>[6x]MDRPAVAGPMDLPIMHDSDRYELVKDIGAGNFGVARLMRDKQANELVAVKYIERGEKIDENVKREIINHRSLRHPNIVRFKEVILTPTHLAIVMEYASGGELFERICNAGRFSEDEARFFFQQLISGVSYAHAMQVAHRDLKLENTLLDGS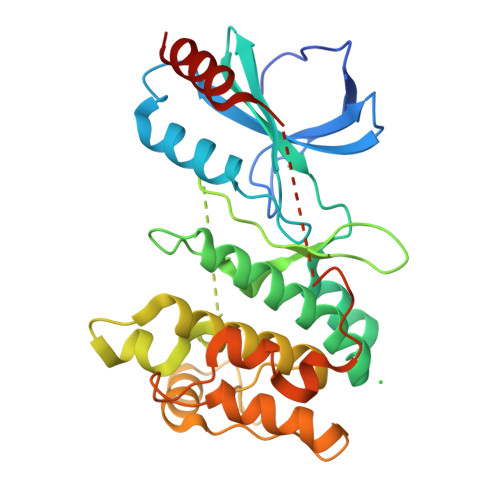PAPRLKIADFGYSKASVLHSQPKSAVGTPAYIAPEVLLKKEYDGKVADVWSCGVTLYVMLVGAYPFEDPEEPKNFRKTIHRILNVQYAIPDYVHISPECRHLISRIFVADPAKRISIPEIRNHEWFLKNLPADLMNDNTMTTQFDESDQPGQSIEEIMQIIAEATV>[3x]GTTSSNSILLKGCDRIVTVVDASTYDAGSAIVSIPITPDIAYRLGSTARTFQRIKYRSLKFRVNAQCATTTAGGYVAGFVKDAADVLPTGTASIPYLMSNTGSFTQPWWKSTVHNVKIPQKLFYTEAPTRGADAVREYCPGQFHVLVDSKPSQICPVTVDLEWVVELHDATFRKESDQTAISAIVADHTLNVYGLPATSNRVGHILISPIGQTPKDLTPTRFATFFGFLPDDKFC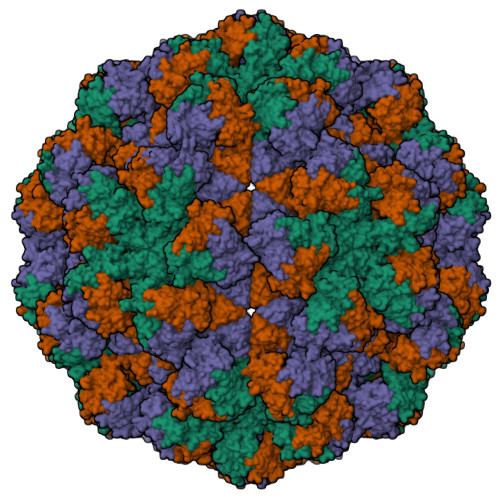VRIPTPVDVVLTGDNVYQSVEATHIRAYLVNGGLGIDFHLAAYNDTTHTIQPIIPTLWNVYDVTGAVTAPFTSAIYDNHVWTHKDKFVPVSFQDEPIPGTVFDYLYPRSYSLPSSNGHHHHHH Zinc-finger antiviral protein (ZAP), also known as poly(ADP-ribose) polymerase 13 (PARP13), is an antiviral factor that selectively targets viral RNA for degradation. ZAP selectively binds CpG dinucleotides through its N-terminal RNA-binding domain, which consists of four zinc fingers. ZAP also contains a central region that consists of a fifth zinc finger and two WWE domains. Through structural and biochemical studies, we found that the fifth zinc finger and tandem WWEs of ZAP combine into a single integrated domain that binds to poly(ADP-ribose) (PAR), a cellular polynucleotide.

PAR binding is mediated by the second WWE module of ZAP and likely involves specific recognition of an adenosine diphosphate-containing unit of PAR. Structural and biochemical analyses revealed that ZAP-CD binds to PAR through the second WWE module. Our data indicate that this ZAP pocket is analogous the isoADPr-binding sites found in other WWE domains. Specifically, we find that the ZAP pocket is configured to accommodate an adenosine diphosphate unit, which is an internal repeating unit of PAR. A single ADP unit without the additional phosphoribose moiety of isoADPr is also found at the free termini of a PAR polymer or in proteins conjugated to a single (mono) ADP-ribose unit (MARylation). However, the ZAP pocket does not fully recapitulate all the structural features of the prototype isoADPr pocket in RNF146, suggesting that there may be differences in binding mode. Moreover, since the composite central domain fold of ZAP has an extended electropositive cleft, we speculate that its ADP pocket may be part of a more extensive binding site for a PAR polymer. Further studies are needed to determine if the ZAP pocket has preference for terminal or internal ADP units of PAR. Mutation of the PAR binding site in ZAP abrogates the interaction in vitro and diminishes ZAP activity against a CpG-rich HIV-1 reporter virus and murine leukemia virus.

> STTSSRVDDHDSEEICLDHLCKGCPLNGSCSKVHFHLPYRWQMLIGKTWTDFEHMETIEKGYCNPGIHLCSVGSYTINFRVMSCDSFPIRRLSTPSSVTKPANSVFTTKWIWYWKNESGTWIQYGEEKDKRKNSNVDSSYLESLYQSCPRGVVPFQAGSRNYELSFQGMIQTNIASKTQKDVIRRPTFVPQWYVQQMKRGPD>[2x]GSMEEEAETEEQQRFSYQQRLKAAVHYTVGCLCEEVALDKEMQFSKQTIAAISELTFRQCENFAKDLEMFARH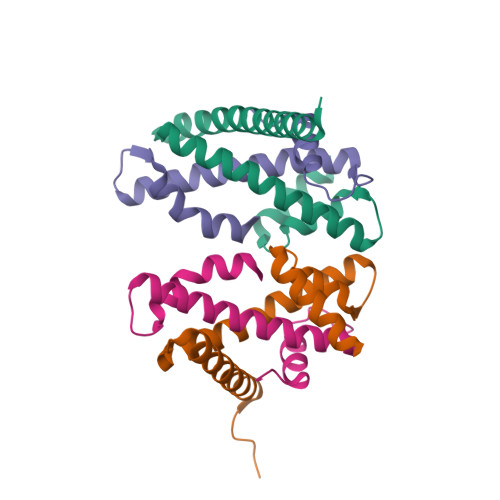AKRTTINTEDVKLLARRSNSLLKYITDKSEEIAQINLER;>GSMEGAGAGSGFRKELVSRLLHLHFKDDKTKVSGDALQLMVELLKVFVVEAAVRGVRQAQAEDALRVDVDQLEKVLPQLLLDF[2x]> GPLGSMASKKVCIVGSGNWGSAIAKIVGGNAAQLAQFDPRVTMWVFEEDIGGKKLTEIINTQHENVKYLPGHKLPPNVVAVPDVVQAAEDADILIFVVPHQFIGKICDQLKGHLKANATGISLIKGVDEGPNGLKLISEVIGERLGIPMSVLMGANIASEVAD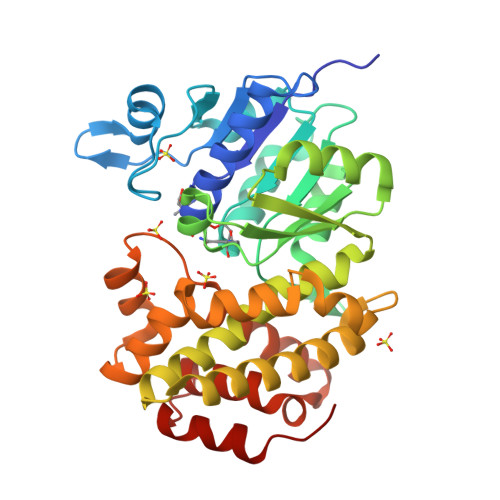EKFCETTIGCKDPAQGQLLKELMQTPNFRITVVQEVDTVEICGALKNVVAVGAGFCDGLGFGDNTKAAVIRLGLMEMIAFAKLFCSGPVSSATFLESCGVADLITTCYGGRNRKVAEAFARTGKSIEQLEKELLNGQKLQGPETARELYSILQHKGLVDKFPLFMAVYKVCYEGQPVGEFIHCLQNHPEHM> GGGCUUCGUUAGGUGAGGCUCCUGUAUGGAGAUACGCU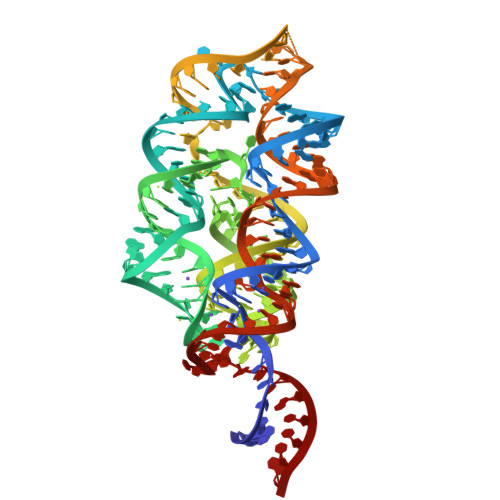GCUGCCCAAAAAUGUCCAAAGACGCCAAUGGGUCAACAGAAAUCAUCGACAUAAGGUGAUUUUUAAUGCAGCUGGAUGCUUGUCCUAUGCCAUACAGUGCUAAAGCUCUACGAUUGAAGCCCA>[2x]HHHHHHMSRLSEPSPYVEFDRRQWRALRMSTPLALTEEELVGLRGLGEQIDLLEVEEVYLPLARLIHLQVAARQRLFAATAEFLGEPQQNPDRPVPFIIGVAGSVAVGKSTTARVLQALLARWDHHPRVDLVTTDGFL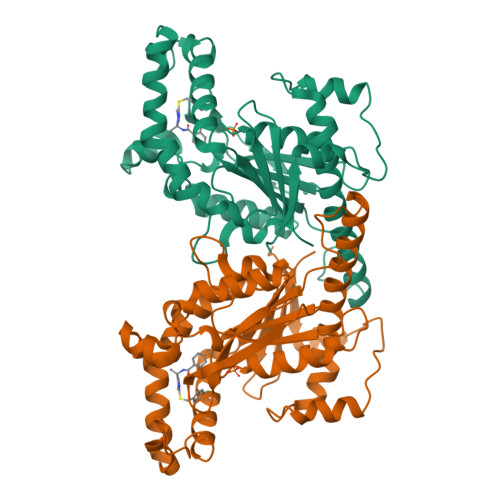YPNAELQRRNLMHRKGFPESYNRRALMRFVTSVKSGSDYACAPVYSHLHYDIIPGAEQVVRHPDILILEGLNVLQTGPTLMVSDLFDFSLYVDARIEDIEQWYVSRFLAMRTTAFADPESHFHHYAAFSDSQAVVAAREIWRTINRPNLVENILPTRPRATLVLRKDADHSINRLRLRKL>MGSSHHHHHHSQENLYFQSQLTTRSKAIASKTKEIEQVYRQDCETFGMVVKMLIEKDPSLEKSIQFALRQ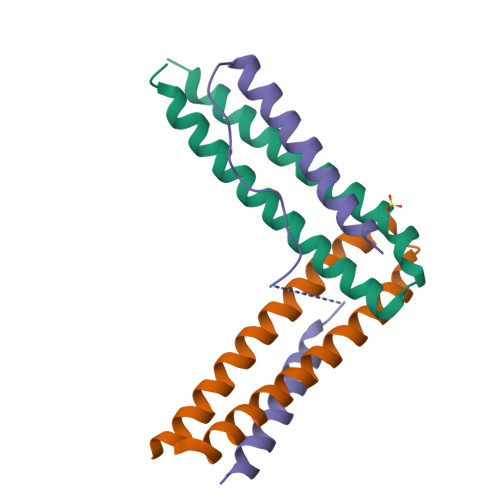NLHEIGERCVEELKHFIAEYDTST[2x];> MSETTERTVLGEYNLFSRKIEEILKQKNVSYVSTVSTPIFSTQEKMKRLSEFIYSKTSKAGVQEFVDGLHEKLNTIIIKASAK>MNLAEKMYKAGQIEFAKGNYETAIIAYTLALLKDPNNAEAWYNLGEAYLALGNYEEAIEAYQKALELDPNNAEAWYNLGEAYLALGDYDNAIEAFTKALELDPNNKTAKAGLKLAKEKKALE[9x];>MTDLS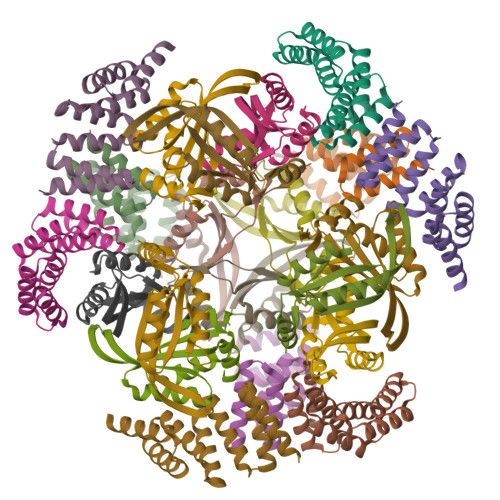SLIETADLRLLLTTVPTETEALYLALAAVEKGLAAEVLITPVTRVRRENGKLVVEDVYRLSFKTTRERLDALVAWLQRRHPLALPECLVLTPIASSVAYRDWLRSSLQGGSHHWGGHHHHHH[12x]>[2x]MAAAASSATISTDSESVSLGHRVRKDFRILHQEVNGSKLVYLDSAATSQKPAAVLDALQNYYEF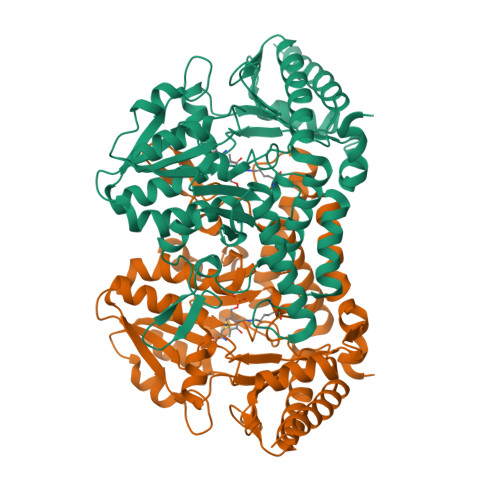YNSNVHRGIHYLSAKATDEFELARKKVARFINASDSREIVFTRNATEAINLVAYSWGLSNLKPGDEVILTVAEHHSCIVPWQIVSQKTGAVLKFVTLNEDEVPDINKLRELISPKTKLVAVHHVSNVLASSLPIEEIVVWAHDVGAKVLVDACQSVPHMVVDVQKLNADFLVASSHKMCGPTGIGFLYGKSDLLHSMPPFLGGGEMISDVFLDHSTYAEPPSRFEAGTPAIGEAIALGAAVDYLSGIGMPKIHEYEVEIGKYLYEKLSSLPDVRIYGPRPSESVHRGALCSFNVEGLHPTDLATFLDQQHGVAIRSGHHCAQPLHRYLGVNASARASLYFYNTKDDVDAFIVALADTVSFFNSFK>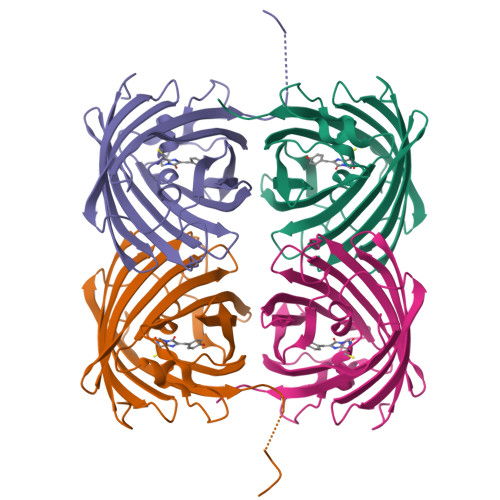GSSHHHHHHSSGLVPGGSHMVSKGEENNMAVIKPDMKIKLRMEGAVNGHPFAIEGVGLGKPFEGKQSMDLKVKEGGPLPFAYDILTTVFCYGNRVFAKYPENIVDYFKQSFPEGYSWERSMNYEDGGICNATNDITLDGDCYIYEIRFDGVNFPANGPVMQKRTVKWEPATEKLYVRDGVLKGDVNTALSLEGGGHYRCDFKTTYKAKKVVQLPDYHFVDHHIEIKSHDKDYSNVNLHEHAEAHSGLPRQAMDELYK[8x]>MGRNEIHKNSLGFGKNDNIYSRNLAQLKLSNYSLLKDSKFESVTEQLTREELYELFDLLVQVPPRTYLLNIWNHKNGICRQGTKDLLKNLRGIAPKLTYRHTGNTNQYGKSPPKITWQGCSYDCNMMVSTLETEQTNRFYNLLNKKAPIDEIKSFIRSCIDEFDKLHTDLYVKYEKIF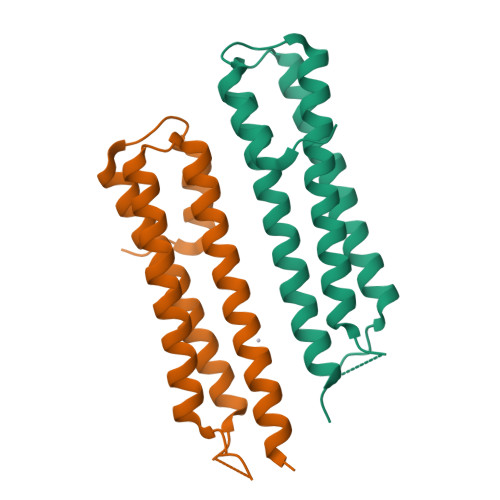SEQKLEHHHHHH[2x]>[2x]MPKNDLLLRSLRGEPIGRFPVWLMRQAGRYMPEYRKIRNRVKNFLELCKNVDLATEISLLPLKILGVDAIIIFSDILVPLEPLGVKVEFVEGEGPKLSWSGKVSDLKKYDPSQNAYVYEIIKRVKEAQDEVPVIGFAGAPFTLLSYLIEGGASKDFKSTKLFMWENPKEYKRLMDILTETVLAYLKEQIKAGADVVQIFDSWVNNLSLEDYGEYVYPYVNYLISELKDFSDTPVIYFFR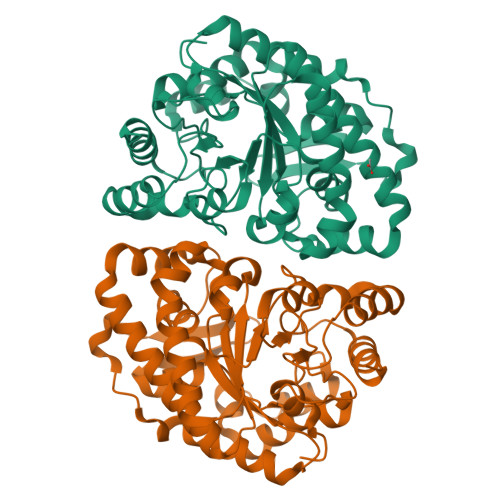GSSSFIDLAVDYRADALSVDWSVDIPELFKIYDKGFQGNLEPAVLYASEEVIEEKTLGLLRRIPVKTRYVFNLGHGLAPDMELEKVKYLVDLVKSFPLT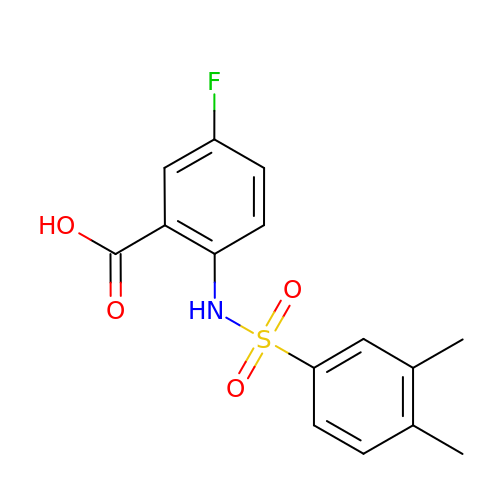2-[(3,4-dimethylphenyl)sulfonylamino]-5-fluoranyl-benzoic acid | C15 H14 F N O4 S | FDKADOFRLAUJSY-UHFFFAOYSA-N>[2x]GPNCAPG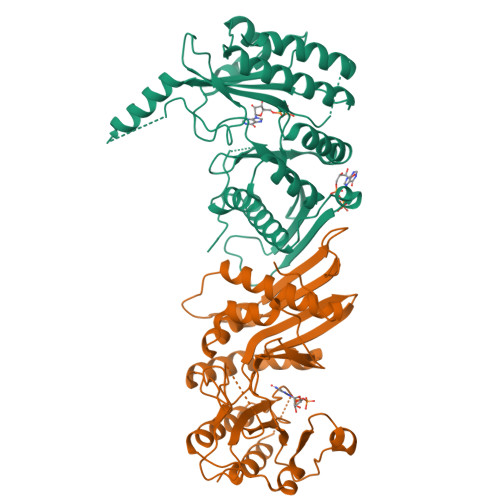QKVKLFRASEPILSVLMWGVNHTINELSNVPVPVMLMPDDFKAYSKIKVDNHLFNKENLPSRFKFKEYCPMVFRNLRERFGIDDQDYQNSVTRSAPINSDSQGRCGTRFLTTYDRRFVIKTVSSEDVAEMHNILKKYHQFIVECHGNTLLPQFLGMYRLTVDGVETYMVVTRNVLSHRLTVHRKYDLKGSTVAREASDKEKAKDLPTFKDNDFLNEGQKLHVGEESKKNFLEKLKRDVEFLAQLKIMDYSLLVGIHDVDRAEQEEMEVEERAEDEECENDGVGGNLLCSYGTPPDSPGNLLSFPRFFGPGEFDPSVDVYAMKSHESSPKKEVYFMAIIDILTPYDTKKKAAHAAKTVKHGAGAEISTVNPEQYSKRFNEFMSNILT>[2x]GMLTYQVKQGDTLNSIAADFRISTAALLQANPSLQAGLTAGQSIVIPGLPDPYTIPYHIAVSIGAKTLTLSLNNRVMKTYPIAVGKILTQTPTGEFYIINRQRN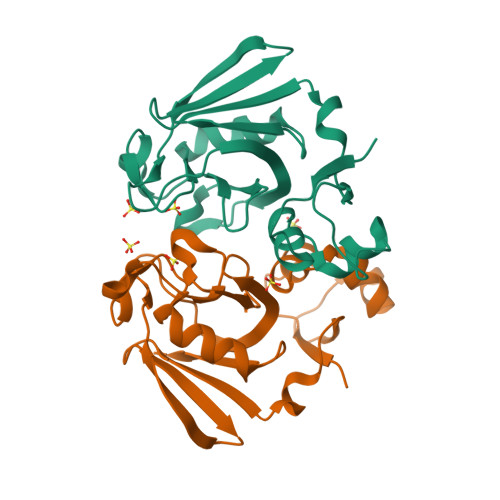PGGPFGAYWLSLSAAHYGIHGTNNPASIGKAVSKGCIRMHNKDVIELASIVPNGTRVTINR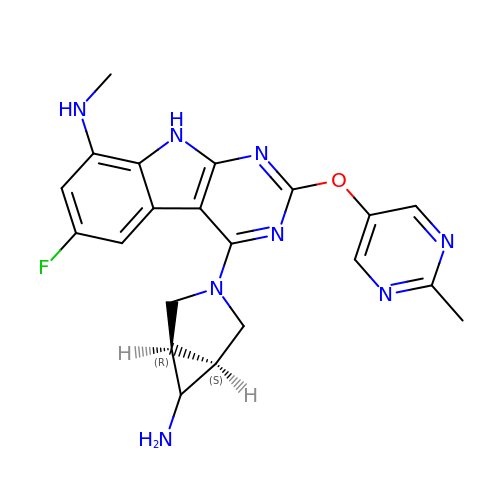4-[(1~{S},5~{R})-6-azanyl-3-azabicyclo[3.1.0]hexan-3-yl]-6-fluoranyl-~{N}-methyl-2-(2-methylpyrimidin-5-yl)oxy-9~{H}-pyrimido[4,5-b]indol-8-amine | C21 H21 F N8 O | GOOKXTQTAFDVNH-HALDLXJZSA-N> GPMDQQNSAVIGQLRLELQQARTEVETADKWRLECIDVCSVLTNRLEE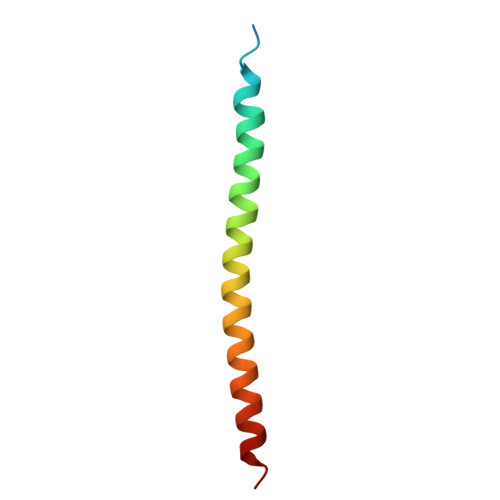EAGFLNSLLK> HHHHHHSSGLVPRGSHMASKIDYLTLFPEMFDGVLNHSIMKRAQENNKLQINTVNFRDYAINKHNQVDDYPYGGGQGMVLKPEPVFNAMEDLDVTEQTRVILMCPQGEPFSHQKAVELSKADHIVFICGHYEGYDERIRTHLVTDEISMGDYVLTGGELPAMTMTDAIVRLIPGVLGNEQSHQDDSFSDGLLEFPQYTRPREFKGLTVPDVLLSGNHANIDAWRHEQKLIRTYNKRPDLIEKYPLTNADKQILERYKIGLKKG

The tRNA m1G37 methyltransferase (TrmD) is considered essential in various bacteria, including Staphylococcus aureus, a pathogen responsible for a wide range of diseases. TrmD was identified as a potentially selective antimicrobial drug target, due to its essential role as well as the structural differences from Trm5. We have identified selective S. aureus TrmD inhibitors with inhibitory activity in the nanomolar to low micromolar range using a direct-to-biology assay read-out. To analyze the binding mode of the compounds identified in the nanoSAR study and to guide future inhibitor optimization, we cocrystallized S. aureus TrmD with inhibitor 2 and the new TrmD inhibitor 8h.

Hill et al. discovered the thienopyrimidone inhibitor 1 by screening a collection of fragments against H. influenzae TrmD, and their subsequent optimization resulted in inhibitor 2 with activities in the nanomolar to micromolar range. The cocrystal structure of 2 was solved at a resolution of 2.5 Å in the space group P4332, containing one protein molecule per asymmetric unit. The N- and C-terminal domains of the monomer were resolved, but the highly flexible linker connecting the domains could not be resolved, similar to many published TrmD structures. ,− For the cocrystallized complex, the N-terminal domain showed discrete electron density for inhibitor 2. Also, the conformation and ligand interactions of 2 were found to be similar for both H. influenzae and S. aureus enzymes. An ionic interaction was formed between the primary amine of 2 and Glu132 in S. aureus (Glu116 in H. influenzae), a residue highly conserved among TrmD orthologues. The thienopyrimidone ring system displayed interactions with S. aureus Met149 (H. influenzae Ile133), Tyr152 (Tyr136), Leu154 (Leu138), and Pro105 (Pro89), within the conserved SAM pocket. To analyze the differences in binding affinity of parent compound 2 between the H. influenzae and S. aureus enzymes, we used the HYDE scoring function in the SeeSAR toolkit to predict favorable and unfavorable contributions of individual ligand atoms to the overall binding energy. The computer-aided investigation revealed that the main difference stems from the amide group interactions, which contributed favorably to H. influenzae TrmD (HYDE: −3.8 kJ/mol), but unfavorably to the S. aureus enzyme (HYDE: +11.0 kJ/mol). Additionally, the terminal amine of inhibitor 2 contributed favorably (HYDE: −3.0 kJ/mol) for the H. influenzae enzyme, whereas it resulted in a slightly unfavorable interaction for the S. aureus enzyme (HYDE: +0.3 kJ/mol). Also, these two crystallographic findings rationalize the results gleaned from the nanoSAR optimization: the transformation of amide to triazole and the transformation of benzylamine to guanidine were beneficial for S. aureus TrmD affinity due to their protein–ligand interactions.>MNHKVHHHHHHIEGRHMPFEIVFDGAKEFADLIATASNLIDEAAFKITEEGVSMRAMDPSRVVLIDLNLPESIFSKYEVEEPETIGINMDHFKKILKRGKSKDTLILRKGDENFLEI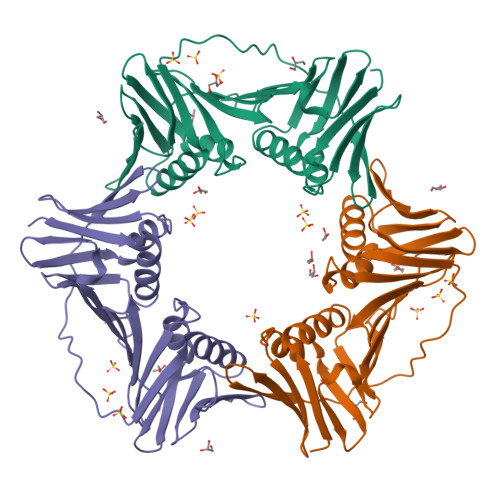TFEGTAKRTFRLPLIDVEELELELPELPFTAKVVLLGEVLKEAIKDASLVSDSLKFIAKEDEFTMKAEGETNEVEIKLTLEDEGLLDLEVEEETRSAYGISYLADMVKGIGKADEVTLRFGTEMPLQMDYFIRDEGKLTFLLAPRVEE[4x]>[2x]GPMEEKALIGIEDFLKVDLRVAKVLSAERVEGSEKLLKLTLSLGDEERTVVAGIAKYYTPEELVGKKIVIVANLKPRKIFGIESQGMILAASDGENLSVIVPDRDVKEGAKLS

Across all domains of life, a widespread class of OB folds have specialized to recognize and manipulate tRNAs, perform key functions in tRNA trafficking and metabolism, and are designated as the tRNA binding domain (TRBD) superfamily (IPR002547; PF01588). In bacteria, Aquifex aeolicus Trbp111 (tRNA-binding protein, 111 amino acids) and Escherichia coli Trbp exemplify the free-standing, dimeric OB-fold proteins that bind diverse tRNA species. Trbp has been suggested to facilitate the folding of the tRNA structure by binding its characteristic elbow region formed by the intercalation of the D-loop into the T-loop and was observed to enhance aminoacylation by several aminoacyl-tRNA synthetases (aaRSs). Contrary to previous proposals, Trbp111 does not recognize the global tRNA structure nor its elbow or anticodon but solely binds its universal 3′ terminal single-stranded CA dinucleotide with a strong positional, structural, and sequence preference.

As described, Trbp111 forms a homodimer where each protomer adopts a canonical OB-fold architecture resembling the Greek key motif, in which five β-strands assemble into two three-stranded β-sheets which are joined to form a β-barrel. The core OB-fold comprises residues 16–89, with the flanking N-terminal (1–15) and C-terminal (90–111) residues of each protomer interacting in an antiparallel manner, forming a central interfacial region. The interface involves an extensive network of hydrogen bonds, salt bridges, hydrophobic interactions, aromatic stacking, and cation-π interactions, altogether burying ~ 1955 Å2 of solvent-accessible surfaces. These contacts produce an unusually robust dimer interface (theoretical ΔG ~ − 22.5 kcal/mol, Kd ~ 3.1 × 10−17 M) that resists denaturation by heat, SDS, Urea, or guanidine treatments. Full denaturation was only achieved when combining heat denaturation and 6 M guanidine treatment. This compact, ultra-stable protein-protein interface is consistent with the hyperthermophilic nature of A. aeolicus, which grows at 85–95 °C. Its resistance to heat and chemical insults is in line with proposed functions as chaperones that may aid the folding of other proteins (e.g., CsaA) or tRNAs (e.g., Trbp). Our Trbp111 apo structure superposes very well with the complex (RMSD ~ 0.6 Å), with key side chains occupying nearly identical positions. Therefore, Trbp111 is pre-organized to capture the terminal CA dinucleotide of tRNAs.1-[[3-[2-oxidanyl-3-(1~{H}-pyrrolo[3,2-c]pyridin-2-yl)phenyl]phenyl]methyl]-3-phenyl-urea 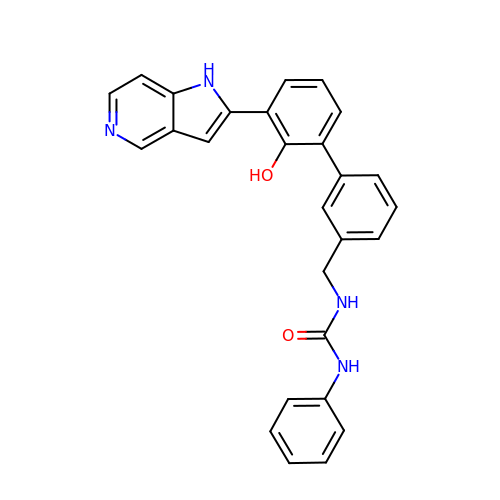| C27 H22 N4 O2 | MYWMHTLQFNYXPC-UHFFFAOYSA-N>SEEVMKDLTSGFIKVLEECKKELNLSESIINDLYNYWKEDYSLLNRDVGCAIVCMSKKLELIDTSG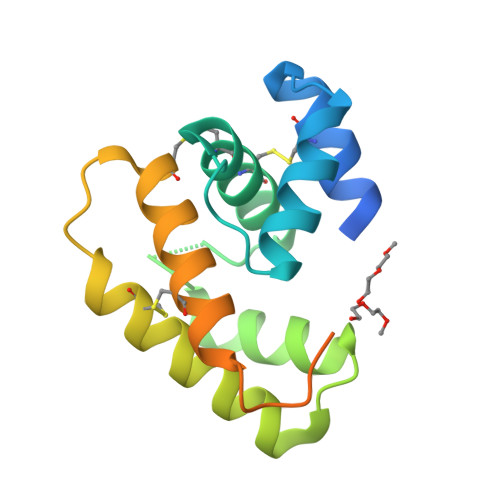KIHHGNAEDLAKKHGADSEVAAKLVAILHECEKTHDAIEDQCMKALEIAKCFRTNIHELNWAPKMDVVITEVLTEVENLYFQGHHHHHHHHHH[2x]(5R,6R)-6-[(1S,2R,4aS,4bS,7R,8aS,10R,10aS)-7,10-dihydroxy-1,2,4b-trimethyltetradecahydrophenanthren-2-yl]-5-methylheptan-2-one 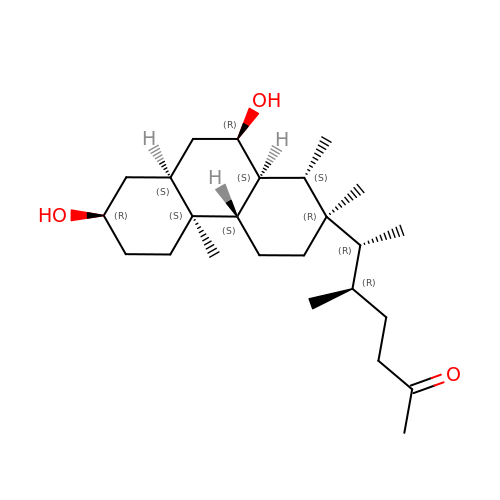| C25 H44 O3 | SZOBNGKCEOANMX-IBSCZREMSA-N>PMFIVNTNVPRASVPDGFLSELTQQLAQATGKPPQYIAVHVVPDQLMAFGGSSEPCALCSLHSIGKIGGAQNRSYSK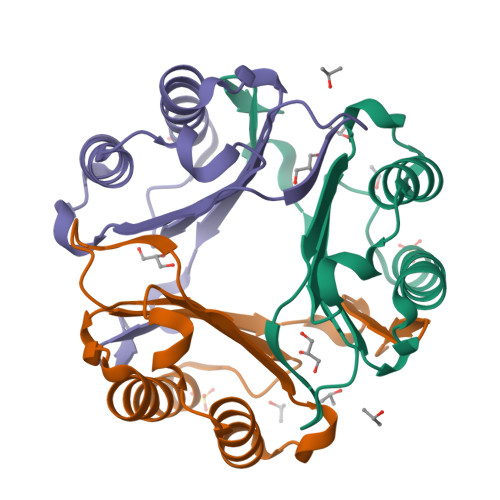LLCGLLAERLRISPDRVYINYYDMNAANVGWNNATFA[3x]>QGGFGNSRGGGAGLGNNQGSNMGGGMNFGEFSINPAMMAA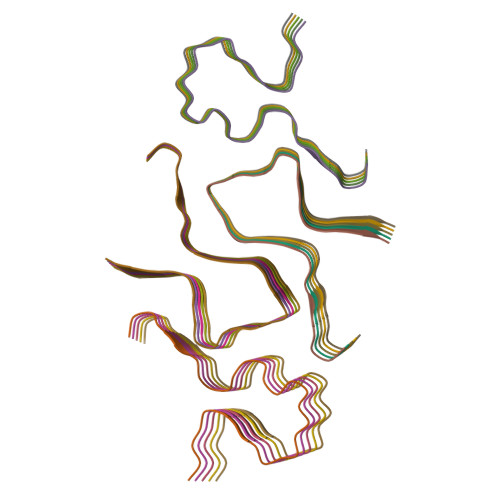AQAALQ[20x]>[2x]MVKITRLTTYRLPPRWMFLKVETDEGVTGWGEPVIEGR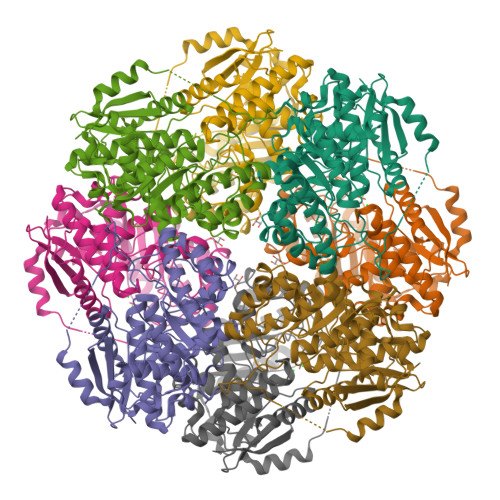ARTVEAAVHELSDYLIGQDPSRINDLWQTMYRAGFYRGGPILMSAIAGIDQALWDIKGKVLGVPVYELLGGLVRDKMRTYSWVGGDRPADVIAGMKALQAGGFDHFKLNGCEEMGIIDTSRAVDAAVARVAEIRSAFGNTVEFGLDFHGRVSAPMAKVLIKELEPYRPLFIEEPVLAEQAETYARLAAHTHLPIAAGERMFSRFDFKRVLEAGGVSILQPDLSHAGGITECVKIAAMAEAYDVALAPHCPLGPIALAACLHVDFVSWNATLQEQSMGIHYNKGAELLDYVRNKADFALEGGYIRPPRLPGLGVDIDEALVIERSKEAPDWRNPVWRHADGSVAEWAENLYFQSHHHHHHWSHPQFEK> QFKDLLLDPLTGDLDFGTPGDRGMRLALTNQLSLRQRL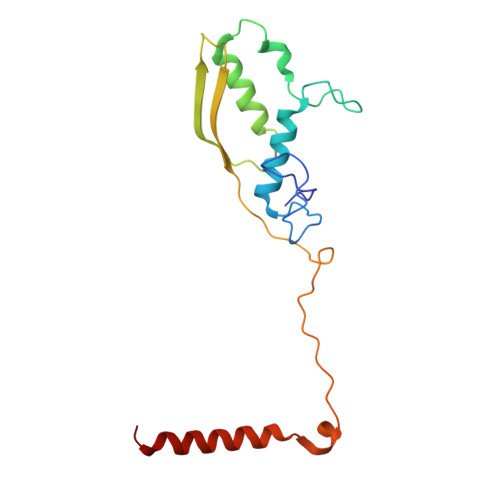YLRFAIWAGDWYFDETFGFPYRTFVGKKTVKAVLDGRIKSEVRQEPDVLQITDFQSTMDVVSRSYKCFFTVVTAEGEEISLAFVGEDEYQYPTPPESNVQLCGDEGVIINFKNKLYYLINFRLPK>GPEKGERISMINPRVVLDENGISHRSRYFIMLCDNETAIAHAKKTSIWAVKKDSSKRISDAYKKASVYFIFVAQQTYNALGYAQVVSDLNSTELPFWSDSSHAGGVRI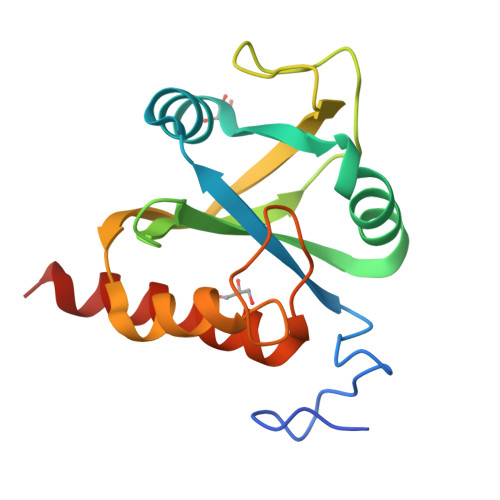KWIKTCNLFSAEISEIVSHMDHGSEARDGMEMMYDEGSRLCTLINYAIMKRIGRDR[2x]> MEQNPQSQLKLLVTRGKEQGYLTYAEVNDHLPEDIVDSDQIEDIIQMINDMGIQVMEEAPDADDLMLAENTADEDAAEAAAQVLSSVESEIGRTTDPVRMYMREMGTVELLTREGEIDIAKRIEDGINQVQCSVAEYPEAITYLLEQYDRVEAEEARLSDLITGFVDPNAEEDLAPTATHVGSELSQEDLDDDEDEDEEDGDDDSADDDNSIDPELAREKFAELRAQYVVTRDTIKAKGRSHATAQEEILKLSEVFKQFRLVPKQFDYLVNSMRVMMDRVRTQERLIMKLCVEQCKMPKKNFITLFTGNETSDTWFNAAIAMNKPWSEKLHDVSEEVHRALQKLQQIEEET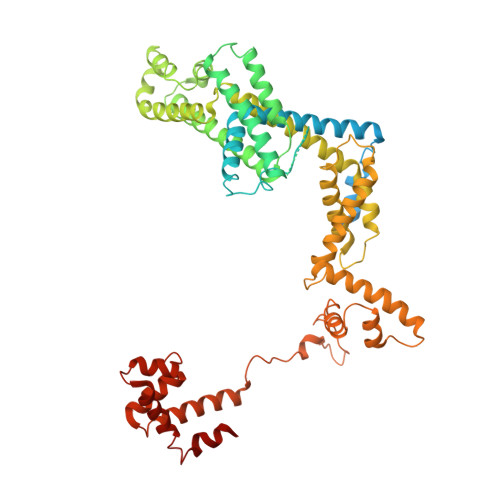GLTIEQVKDINRRMSIGEAKARRAKKEMVEANLRLVISIAKKYTNRGLQFLDLIQEGNIGLMKAVDKFEYRRGYKFSTYATWWIRQAITRSIADQARTIRIPVHMIETINKLNRISRQMLQEMGREPTPEELAERMLMPEDKIRKVLKIAKEPISMETPIGDDEDSHLGDFIEDTTLELPLDSATTESLRAATHDVLAGLTAREAKVLRMRFGIDMNTDYTLEEVGKQFDVTRERIRQIEAKALRKLRHPSRSEVLRSFLDD> YVDYKDDDDKEFMHSFCAFKADDGPCRACMKRFFFNIFTRQC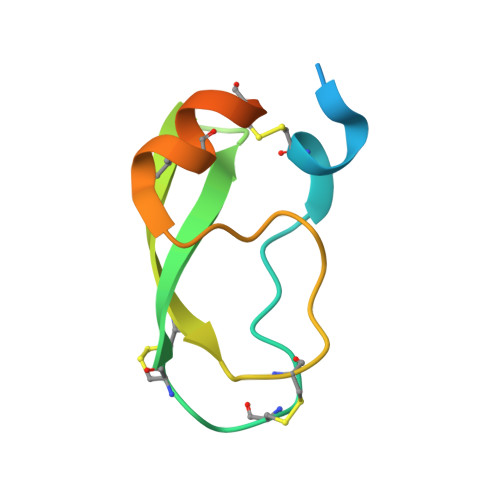EEFCYGGCEGNQNRFESLEECKKMCTRDPRHHHHHHAN> GPGGSGGVTEEQVHHIVKDALQRYSEDRIGLADYALESGGASVISTRCSETYETKTALISLFGIPLWYHSQSPRVILQPDVHP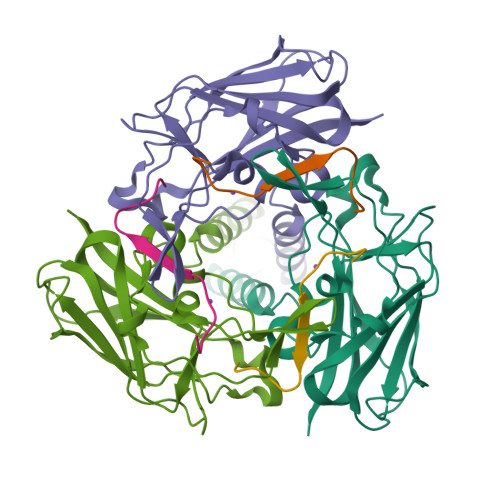GNCWAFQGPQGFAVVRLSARIRPTAVTLEHVPKALSPNSTISSAPKDFAIFGFDEDLQQEGTLLGKFTYDQDGEPIQTFHFQAPGRGTYQVVELRILTNWGHPEYTCIYRFRVHGEPAH;> GPGGSGEEDRSCTLANNFARSFTLMLRYNGPPPT> MTRCLMFTLLFLVSSLISTVGLPVEPPAELLQLGGGDVGGGRLSVDASDIAEASRDFGGVARAEPMAVFHPRAAGDVAGLVGAAFRSARGFRVSARGHGHSISGQAQAAGGVVVDMSRGRGPGAAVARALPVHSAALGGHYVDVWGGELWVDVLNWTLSHGGLAPRSWTDYLYLSVGGTLSNAGISGQAFHHGPQISNVYELDVVTGKGEVVTCSETENPDLFFGVLGGLGQFGIITRARIALERAPKRVRWIRALYSNFSEFTADQERLISLGSGGGRRFDYVEGFVVAAEGLINNWRSSFFSPQNPVKLTSLKHHSSVLYCLEVTKNYDDE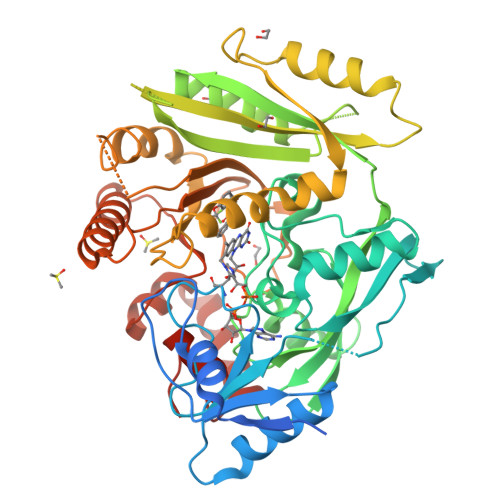TAGSVDQDVDTLLGELNFLPGTVFTTDLPYVDFLDRVHKAELKLRAKGMWEVPHPWLNLFVPASRIADFDRGVFRGVLGGRTAGAGGPVLIYPMNKHKWDPRSSAVTPDEEVFYLVAFLRSALPGAPESLEALARQNQRILDFCAGTGIGAKQYLPGHKARHEWAEHFGAARWDRFARLKAEFDPRAILAAGQGIFRPPGSPALAADS> MRAHRIDTFLIRENIKLEIIHESNSYFGGEHISIAFRFKHLGSQHELFNYKEKLLTVDKAVEEKLEQQAKVQDDGEGTMENQTWSLKSLLGAFKRTGEPEESVDVDNMKMLNESKMLREKIQKQMYFHQPVTLISGYVQISGVFQYDSEVISESKFKQDEVKMVGLDIVPGHTTNSVLALEDGEHFKGKRNLTNYLNSDYTNVTNGLLFSESGSRGRTGTYNERTLMISNDTSIKTLPLLLIPQTLLFSEISLEPGEVRTFYFKSTKLPKDICPSYSSSKVASINYTLEVGADVLSDDNIEKFSNRVPITIAPYISSNAEQYTSRLDKPAIILKTGNIKELKPRLFTRKVSTASAVSFGRRKSSIIDIDSPLEDNEFVXXXXXXXXXXXXSNQNVSRXXXXXXXXXXXXQFGKDEDSSDPEPNDSHFSNEMVTSAESSLRSDAVTKRRKSYSVRDNISNLEQKMWNDCSLVKSDENSNLLPQLINLQNAYQINRNNETMAKVSLSAPFYKTTDDINLVIELDPITTPLLKVTSLTVSLESFEIINPKYKTEG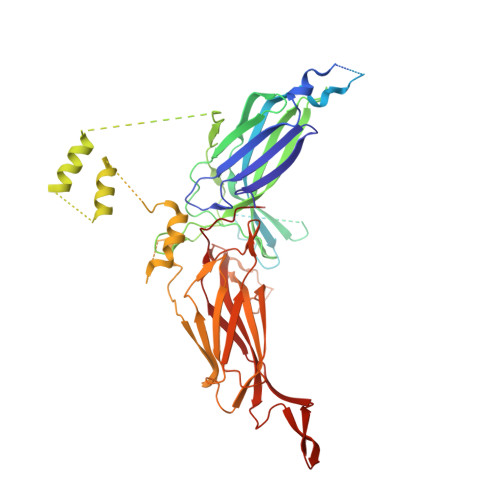KGIGSKPKGNSVYEKHFICFDECKSVSVKLLPPRSPTNQITGQFKTDVFQHKWMIGLKFVIIAKTESITLDQFYEDKKGILFHSKENLEGEEFTCYVPIPILCTSEDFMGW>MGDKPIWEQIGSSFIQHYYQLFDNDRTQLGAIYIDASCLTWEGQQFQGKAAIVEKLSSLPFQKIQHSITAQDHQPTPDSCIISMVVGQLKA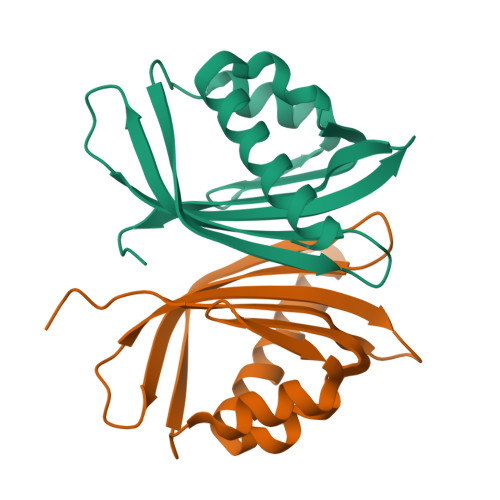NENPIMGFHQMFLLKNINDAWVCTNDMFRLALHNFG[2x]>TERLAGKTALVTGAAQGIGKAIAARLAADGATVIVSDINAEGAKAAAASIGKKARAIAADISDPGSVKALFAEIQALTGGIDILVNNASIVPFVAWDDVDLDHWRKIIDVNLTGTFIVTRAGTDQMRAAGKAGRVISIASNTFFAGTPNMAAYVAAKGGVIGFTRALATELGKYNITANAVTPGLIESDGVKASPHNEAFGFVEMLQAMKGKGQPEHI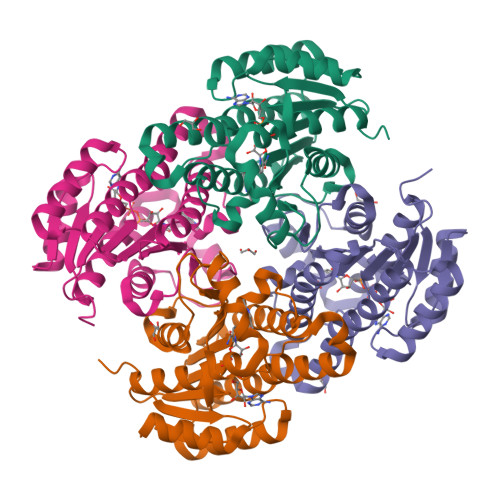ADVVSFLASDDARWITGQTLNVDAGMVRH[4x]>GAMGSGASSQAACLKQILLLQLDLIEQQQQQLQAKEKEIEELKS[2x]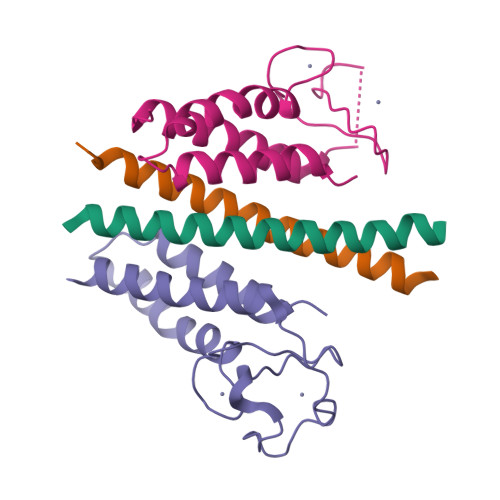;>MNPVNATALYISASRLVLNYDPGDPKAFTEINRLLPYFRQSLSCCVCGHLLQDPIAPTNSTCQHYVCKTCKGKKMMMKPSCSWCKDYEQFEENKQLSILVNCYKKLCEYITQTTLA[2x]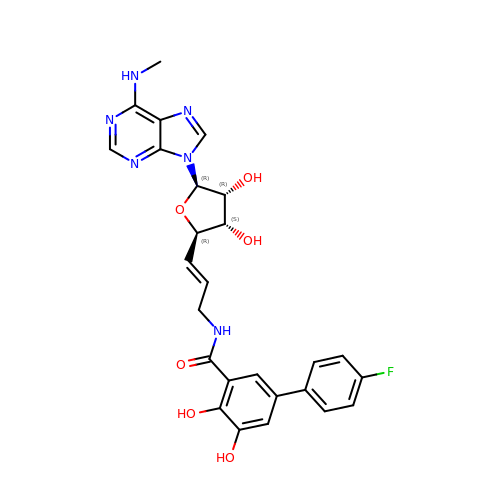N-[(E)-3-[(2R,3S,4R,5R)-3,4-dihydroxy-5-(6-methylaminopurin-9-yl)oxolan-2-yl]prop-2-enyl]-5-(4-fluorophenyl)-2,3-dihydroxy-benzamide | C26 H25 F N6 O6 | NSQDVYXOGVOLPV-WKWRZTKWSA-N>[4x]MSLAHPPRLNDDKPVIWTVSVTRLFELFRDISLEFDHLANITPIQLGFEKAVTYIRKKLANERCDAI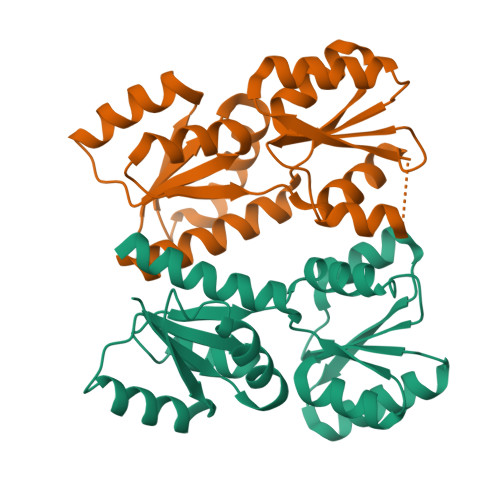IAAGSNGAYLKSRLSVPVILIKPSGYDVLQFLAKAGKLTSSIGVVTYQETIPALVAFQKTFNLRLDQRSYITEEDARGQINELKANGTEAVVGAGLITDLAEEAGMTGIFIYSAATVRQAFSDALDMTRMSLRHNTHDATRNALRTRYVLEGHHHHHH N-SUCCINYL PHENYLGLYCINE | C12 H13 N O5 | 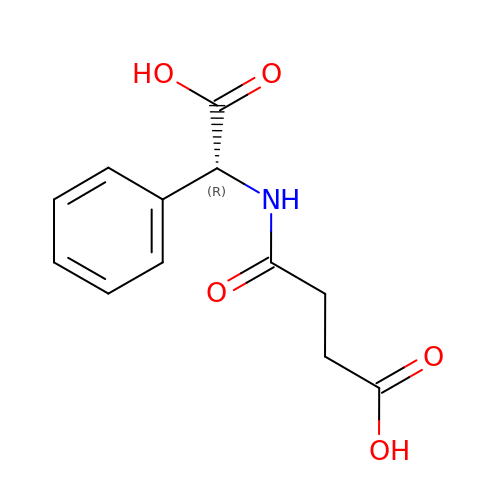GQFHIYFXQQEWME-LLVKDONJSA-N6-(2,3,4,5,6,7-HEXAHYDRO-2,4,4-TRIMETHYL-1-METYLENEINDEN-2-YL)-3-METHYLHEXA-2,4-DIENOIC ACID | C20 H28 O2 | 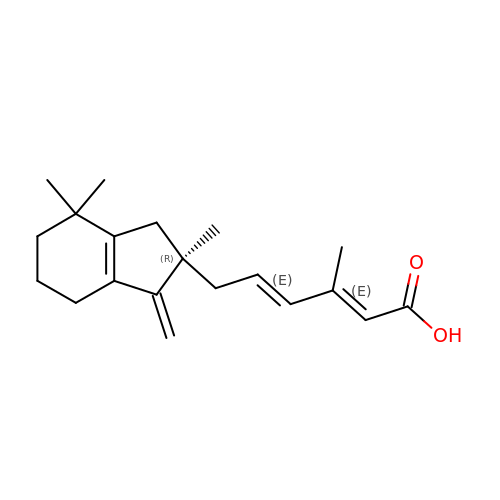HEVXQLBAMFMFKU-IAZPEVBMSA-N> SMATSNLLKNKGSLQFEDKWDFMRPIVLKLLRQESVTKQQWFDLFSDVHAVCLWDDKGPAKIHQALKEDILEFIKQAQARVLSHQDDTALLKAYIVEWRKFFTQCDILPKPFCQLEITLMGKQGSNKKSNVEDSIVRKLMLDTWNESIFSNIKNRLQDSAMKLVHAERLGEAFDSQLVIGVRESYVNLCSNPEDKLQIYRDNFEKAYLDSTERFYRTQAPSYLQQNGVQNYMKYADAKLKEEEKRALRYLETRRECNSVEALMECCVNALVTSFKETILAECQGMIKRNETEKLHLMFSLMDKVPNGIEPMLKDLEEHIISAGLADMVAAAETIT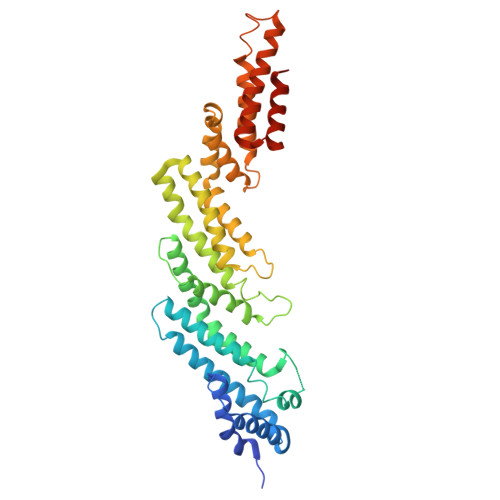TDSEKYREQLDTLFNRFSKLVKEAFQDDPRFLTARDKAYKAVVNDATIFKLE> SMEQDIFLWRKETGFGFRILGGNEPGEPIYIGHIVP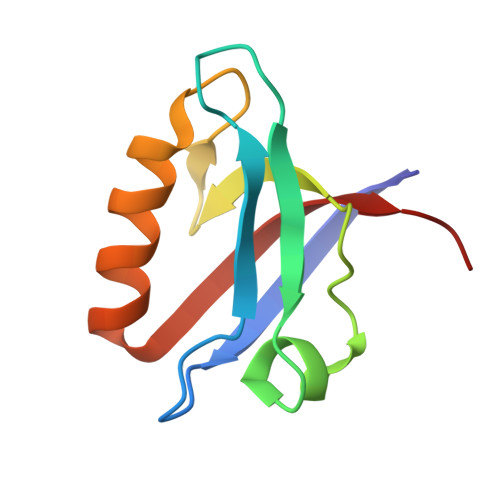LGAADTDGRLRSGDELISVDGTPVIGKSHQLVVQLMQQAAKQGHVNLTVRQTRL>[7x]MHLPQMGYDRAITVFSPDGRLFQVEYAREAVKRGATAIGIKCKEGVILIADKRVGSKLLEKDTIEKIYKIDEHICAATSGLVADARVLIDRARIEAQINRLTYDIPITVKELAKKICDF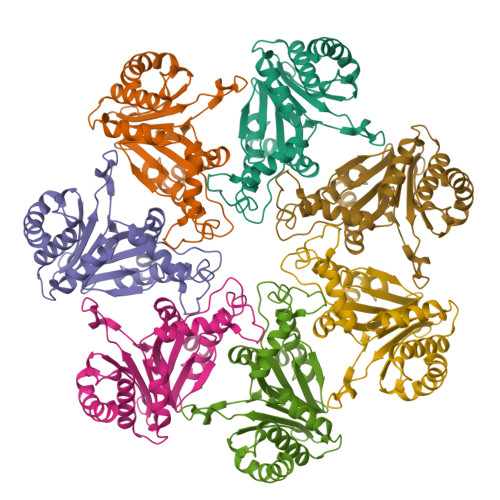KQQYTQYGGVRPFGVSLLIAGVNEVPKLYETDPSGALLEYKATAIGMGRMAVTEFFEKEYRDDLSFDDAMVLGLVAMGLSIESELVPENIEVGYVKVDDRTFKEVSPEELKPYVERANERIRELLKK>[3x]GAMGWCIFIYNLGQDADEGILWQMFGPFGAVTNVKVIRDF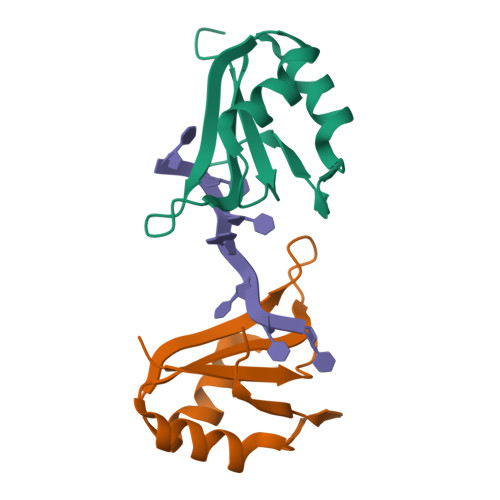NTNKCKGFGFVTMTNYEEAAMAIASLNGYRLGDKILQVSFKTNKSHK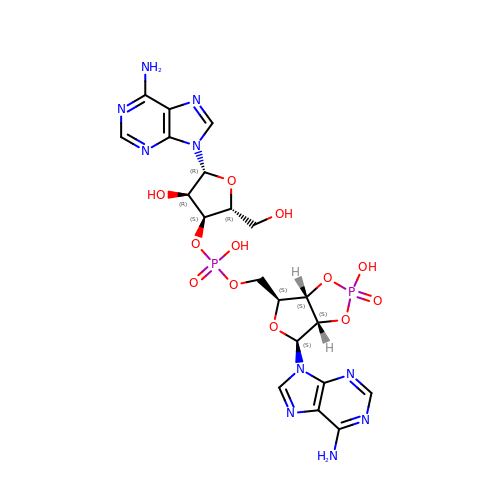3'-O-[(R)-{[(2S,3aS,4S,6S,6aS)-6-(6-amino-9H-purin-9-yl)-2-hydroxy-2-oxotetrahydro-2H-2lambda~5~-furo[3,4-d][1,3,2]dioxaphosphol-4-yl]methoxy}(hydroxy)phosphoryl]adenosine | C20 H24 N10 O12 P2 | ZKDCIJKZCQKMKS-RJLGOGMOSA-N2-(6-HYDROXY-1,3-BENZOTHIAZOL-2-YL)-1,3-THIAZOL-4(5H)-ONE 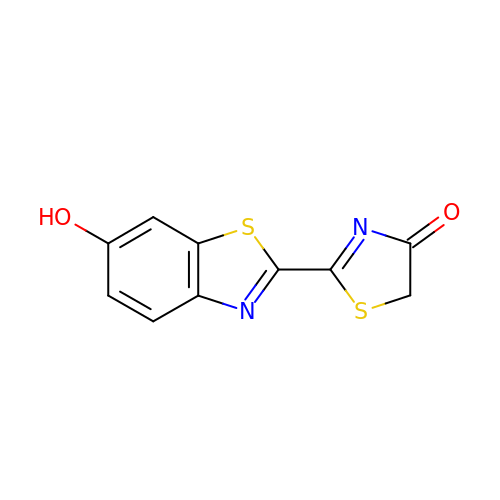| C10 H6 N2 O2 S2 | JJVOROULKOMTKG-UHFFFAOYSA-N>MKRFFNRFYLDTGIIADPSQRSLASRVSAFLVQGAVAFSLLGTIGVDTSPLIAAAGVTGATIGFALKDFGTNFVASIVLSGQQSIRTGNLVCIGTGLNVVKGKVVDWDTRYLYLRSSEGHLLHVPNNMVLNSVVTWEQEKKQNPHETDLPKQ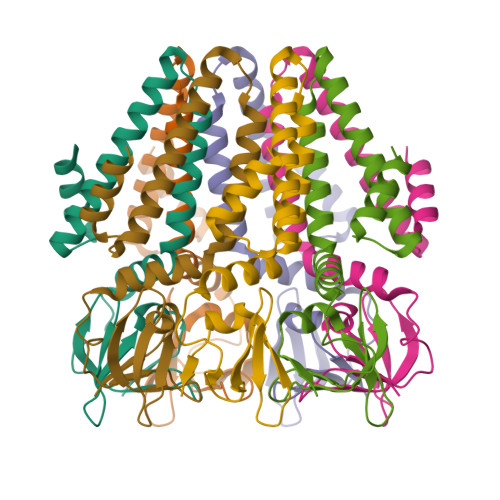DVVKAPGDNAAKQSNSLEVLFQ[7x]>[2x]RDQEQYIHRKCYQEFAHCYLVKYKTPQPWPNEGLIADQCPLPGLADVSFYPYQAIWDYYAKIENIRPANWTSSKLYGKARMGSYYIPKRLRNINNTHILFCSDVLYSKWYNLQNSILQNENELTKRLSNLTIGNKLKNRALPYEWAKGGLNRLFRNISVLDVCSRPEMVLLLNKTYYTFSLWEGDCNITRYNVNETVPECKDFPHRRFNDHPYSCRLWRYREGKEEVKCLTSDHTRCLYYPEYSNPEALFDFGFLSYMRNFPGPQCIESTSIRQQDYEVYSIYQECKLASKTYGIDSVLFSLKNFLNYTGKPVNEMPNARAFVGLIDPKFPPTYPDDDDK

The FV envelope (Env) glycoprotein belongs to a class I fusogens, which are synthesized as single-chain precursors that fold into trimers, and whose protomers are subsequently cleaved in the Golgi compartment during transport to the cell surface. FV Env is cleaved at two sites by cellular furin during maturation, giving rise to 3 fragments: the leader peptide (LP), the surface (SU) subunit, which includes the receptor-binding domain (RBD), and the transmembrane subunit (TM), which harbors the fusion machinery. In this manuscript we present the X-ray structure of the RBD from a zoonotic gorilla FV at 2.57 Å resolution, which reveals a novel fold. We identified, within the RBD, two subdomains in terms of their structure, conservation, and function: the upper subdomain, which encompasses most of the genotype-specific region, and a more conserved, lower subdomain, important for binding to the attachment factor HS.

Recombinant RBDs from several simian FV (SFV) strains were tested for production in Drosophila S2 insect cells, and only the RBD from gorilla SFV (strain SFVggo_huBAK7422, genotype II; abbreviated as ‘GII’ herein) was expressed in high enough yields and formed crystals. Crystals were obtained for the RBDD, as well as for the untreated protein (RBDG). The RBDD diffracted better (2.57 Å) than RBDG (2.80 Å) and the structural analyses presented below were carried out using the RBDD structure, unless otherwise noted. The NAG and MAN units built only into the RBDG (and not RBDD) structure are indicated with red frames. A prominent feature of the upper subdomain is the eighth N-linked sugar (N8)18 attached to the α4 helix residue N390. The N390 side chain and the first two attached NAG residues are buried in the RBD, rendering the EndoH/D cleavage site inaccessible, which allowed building 10 sugar residues in RBDG and 8 in the deglycosylated protein crystals. The N8 glycan emerges from a cavity that has N390 at its base and extends upwards, remaining in contact with the protein and preserving the same conformation in both crystal forms. Structural analyses revealed that the glycan establishes extensive van der Waal contacts with the residues underneath (buried surface area of 803 Å2) and forms hydrogen bonds with main-chain atoms from Y394 and I484 and the side chain of E361. N8 is the only N-glycosylation site in SU that is strictly conserved across the FV subfamily, and the hydrophobic patch residues laying beneath it are conserved as well.> MKTLADALKEFEVLSFEIDEQALAFDVDNIEMVIEKSDITPVPKSRHFVEGVINLRGRIIPVVNLAKILGISFDEQKMKSIIVARTKDVEVGFLVDRVLGVLRITENQLDLTNVSDKFGKKSKGLVKTDGRLIIYLDIDKIIEEI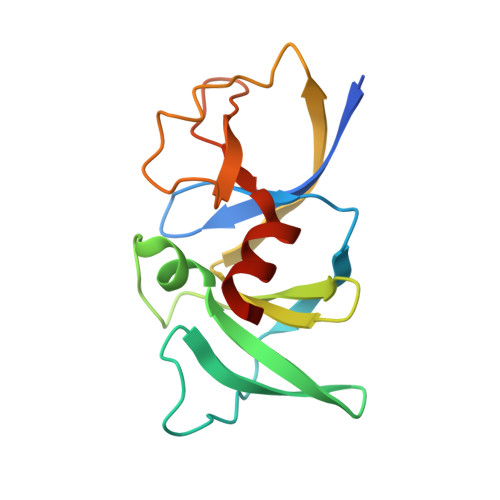TVKEGV>[4x]FDYDGPLMKTEVPGPRSRELMKQLNIIQNAEAVHFFCNYEESRGNYLVDVDGNRMLDLYSQISSIPIGYSHPALVKLVQQPQNVSTFINRPALGILPPENFVEKLRESLLSVAPKGMS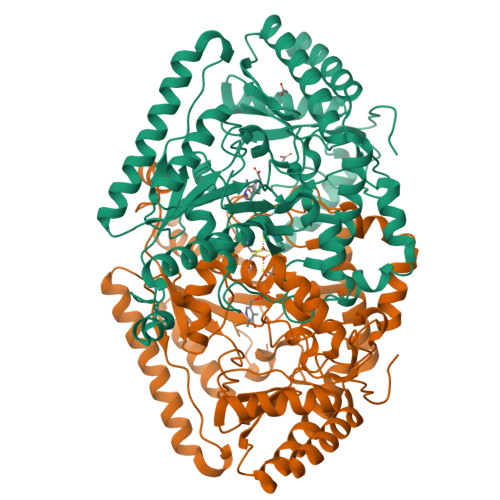QLITMACGSCSNENAFKTIFMWYRSKERGESAFSKEELETCMINQAPGCPDYSILSFMGAFHGRTMGCLATTHSKAIHKIDIPSFDWPIAPFPRLKYPLEEFVKENQQEEARCLEEVEDLIVKYRKKKKTVAGIIVEPIQSEGGDNHASDDFFRKLRDISRKHGCAFLVDEVQTGGGSTGKFWAHEHWGLDDPADVMTFSKKMMTGGFFHKEEFRPNAPYRIFNTWLGDPSKNLLLAEVINIIKREDLLSNAAHAGKVLLTGLLDLQARYPQFISRVRGRGTFCSFDTPDESIRNKLISIARNKGVMLGGCGDKSIRFRPTLVFRDHHAHLFLNIFSDILADFA>[8x]MSKAGASL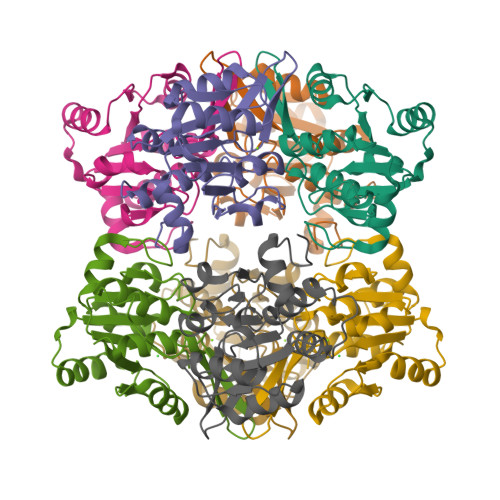ATCYGPVSADVMAKAENIRLLILDVDGVLSDGLIYMGNNGEELKAFNVRDGYGIRCALTSDIEVAIITGRKAKLVEDRCATLGITHLYQGQSNKLIAFSDLLEKLAIAPENVAYVGDDLIDWPVMEKVGLSVAVADAHPLLIPRADYVTRIAGGRGAVREVCDLLLLAQGKLDEAKGQSI>AAVILESIFLKRSQQKKKTSPLNFKKCLFLLTVHKLSYYEYDFERGRRGSKKGSIDVEKITCVETVVPEKNPPPERQIPRRGEESSEMEQISIIERFPYPFQVVYDEGPLYVFSPTEE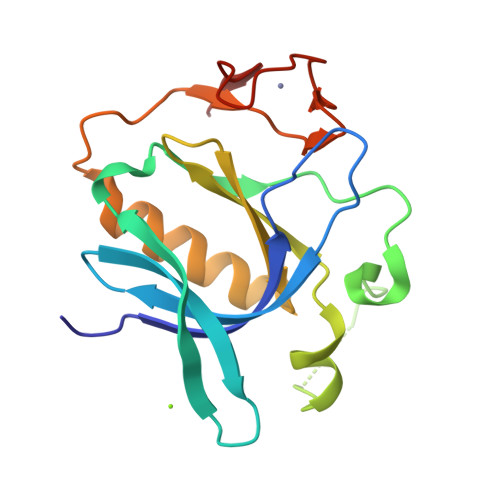LRKRWIHQLKNVIRYNSDLVQKYHPCFWIDGQYLCCSQTAKNAMGCQILEN[2x]(1R,3R,7E,17beta)-17-[(2R)-5-hydroxy-5-methylhexan-2-yl]-2-methylidene-9,10-secoestra-5,7-diene-1,3-diol 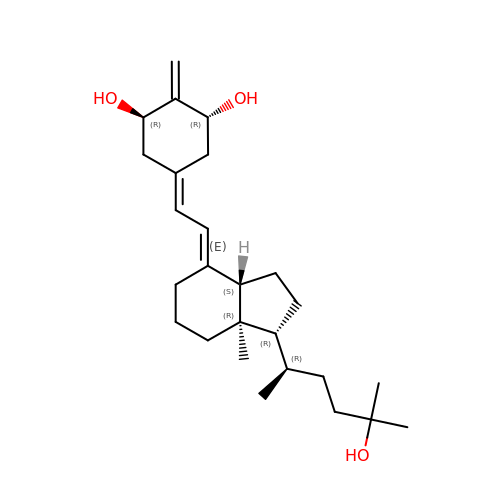| C26 H42 O3 | JLJBOAPFTSKXIR-PXIOBPQKSA-N>[4x]MHHHHHHSTPSIVIASAARTAVGSFNGAFANTPAHELGATVISAVLERAGVAAGEVNEVILGQVLPAGEGQNPARQAAMKAGVPQEATAWGMNQLCGSGLRAVALGMQQIATGDASIIVAGGMESMSMAPHCAHLRGGVKMGDFKMIDTMIKDGLTDAFYGYHMGTTAENVAKQWQLSRDEQDAFAVASYNKAEAAQKDGRFKDEIVPFIVKGRKGDITVDADEYIRHGA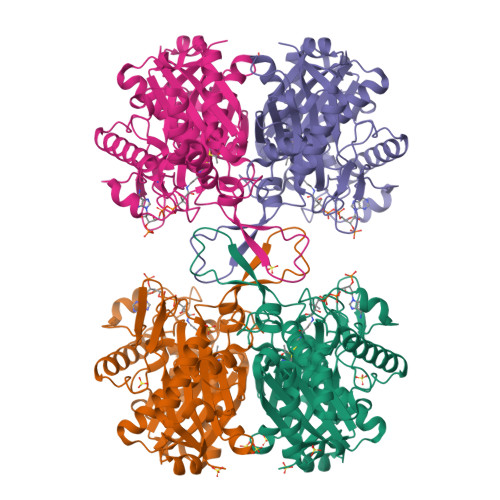TLDSMAKLRPAFDKEGTVTAGNASGLNDGAAAALLMSEAEASRRGIQPLGRIVSWATVGVDPKVMGTGPIPASRKALERAGWKIGDLDLVEANEAFAAQACAVNKDLGWDPSIVNVNGGAIAIGHPIGASGARILNTLLFEMKRRGARKGLATLCIGGGMGVAMCIESL> MVSTYDEIEIEDMTFEPENQM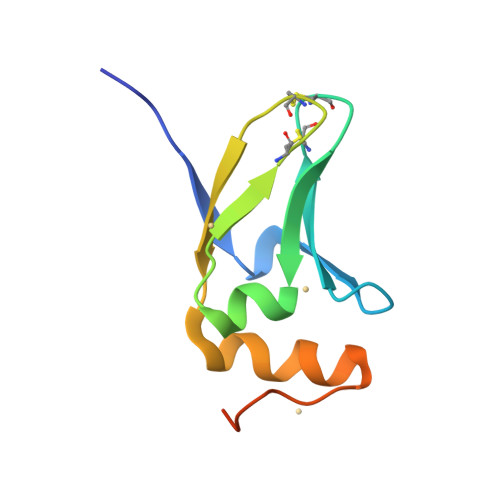FTYPCPCGDRFQIYLDDMFEGEKVAVCPSCSLMIDVVFDKEDLAEYYEEAGIHPPEPIAAAAHHHHHH>[2x]NAQFLHTQVGRGLLGAVVNPLGEVTDKFA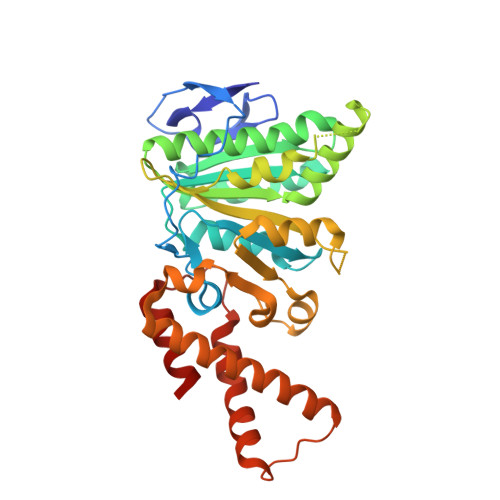VTDNSEILYRPVDNAPPLYSERAAIEKPFLTGIKVIDSLLTCGEGQRMGIFASAGCGKTFLMNMLIEHSGADIYVIGLIGERGREVTETVDYLKNSEKKSRCVLVYATSDYSSVDRCNAAYIATAIAEFFRTEGHKVALFIDSLTRYARALRDVALAAGESPAARGYPVSVFDSLPRLLERPGKLKAGGSITAFYTVLLEDDDFADPLAEEVRSILDGHIYLSRNLAQKGQFPAIDSLKSISRVFTQVVDEKHRIMAAAFRELLSEIEELRTIIDFGEYKPGENASQDKIYNKISVVESFLKQDYRLGFTYEQTMELIGETIR>[3x]GPDEEPEEPGRRGSFVEMVDNLRGKSGQGYYVEMTVGSPPQTLNILVDTGSSNFAVGAAPHPFLHRYYQRQLSSTYRDLRKGVYVPYTQGKWEGELGTDLVSIPHGPNVTVRANIAAITESDKFFINGSNWEGILGLAYAEIARPDDSLEPFFDSLVKQTHVPNLFSLQLCGAGFPLNQSEVLASVGGSMIIGGIDHSLYTGSLWYTPIRREWYYEVIIVRVEINGQDLKM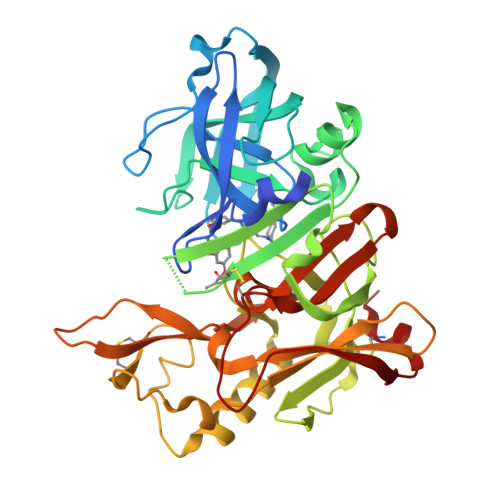DCKEYNYDKSIVDSGTTNLRLPKKVFEAAVKSIKAASSTEKFPDGFWLGEQLVCWQAGTTPWNIFPVISLYLMGEVTNQSFRITILPQQYLRPVEDVATSQDDCYKFAISQSSTGTVMGAVIMEGFYVVFDRARKRIGFAVSACHVHDEFRTAAVEGPFVTLDMEDCGYNI>[4x]GSMSAKD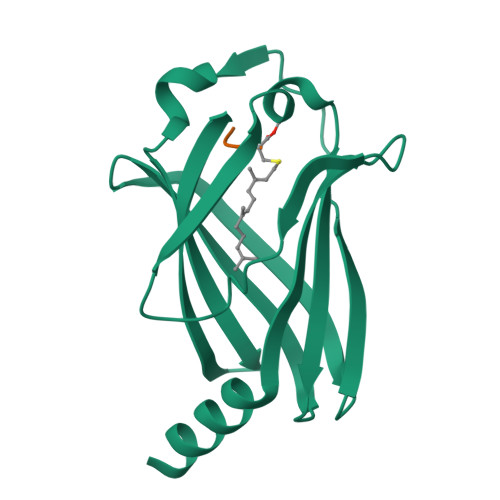ERAREILRGFKLNWMNLRDAETGKILWQGTEDLSVPGVEHEARVPKKILKCKAVSRELNFSSTEQMEKFRLEQKVYFKGQCLEEWFFEFGFVIPNSTNTWQSLIEAAPESQMMPASVLTGNVIIETKFFDDDLLVSTSRVRLFYV;>CSQQGKSSC[2x]> MKTRIHVVQGDITKLAVDV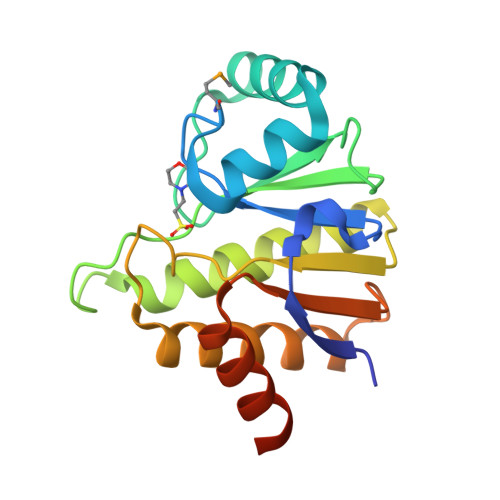IVNAANPSLMGGGGVDGAIHRAAGPALLDACLKVRQQQGDCPTGHAVITLAGDLPAKAVVHTVGPVWRGGEQNEDQLLQDAYLNSLRLVAANSYTSVAFPAISTGVYGYPRAAAAEIAVKTVSEFITRHALPEQVYFVCYDEENAHLYERLLTQQGDEEHHHHHH>MNCVCRLVLVVLSLWPDTAVAPGPPPGPPRVSPDPRAELDSTVLLTRSLLADTRQLAAQLRDKFPADGDHNLDSLPTLAMSAGALGALQLPGVLTRLRADLLSYLRHVQWLRRAGGSSLKTLEPELGTLQARLDRLLRRLQLLMSRLALPQPPPDPPAPPLAPPSSAWGGIRAAHAILGGLHLTLDWAVRGLLLLKTRL[2x];>MSSSCSGLSRVLVAVATALVSASSPCPQAWGPPGVQYGQPGRSVKLCCPGVTAGDPVSWFRDGEPKLLQGPDSGLGHELVLAQADSTDEGTYICQTLDGALGGTVTLQLGYPPARPVVSCQAADYENFSCTWSPSQISGLPTRYLTSYRKKTVLGADSQRRSPSTGPWPCPQDPLGAARCVVHGAEFWSQYRINVTEVNPLGASTRLLDVSLQSILRPDPPQGLRVESVPGYPRRLRASWTYPASWPCQPHFLLKFRLQYRPAQHPAWSTVEPAGLEEVITDAVAGLPHAVRVSARDFLDAGTWSTWSPEAWGTPSTGTIPKEIPAWGQLHTQPEVEPQVDSPAPPRPSLQPHPRLLDHRDSVEQVAVLASLGILSFLGLVAGALALGLWLRLRRGGKDGSPKPGFLASVIPVDRRPGAPNL[2x];>[2x]MSAPRIWLAQALLFFLTTESIGQLLEPCGYIYPEFPVVQRGSNFTAICVLKEACLQHYYVNASYIVWKTNHAAVPREQVTVINRTTSSVTFTDVVLPSVQLTCNILSFGQIEQNVYGVTMLSGFPPDKPTNLTCIVNEGKNMLCQWDPGRETYLETNYTLKSEWATEKFPDCQSKHGTSCMVSYMPTYYVNIEVWVEAENALGKVSSESINFDPVDKVKPTPPYNLSVTNSEELSSILKLSWVSSGLGGLLDLKSDIQYRTKDASTWIQVPLEDTMSPRTSFTVQDLKPFTEYVFRIRSIKDSGKGYWSDWSEEASGTTYEDRPSRPPSFWYKTNPSHGQEYRSVRLIWKALPLSEANGKILDYEVILTQSKSVSQTYTVTGTELTVNLTNDRYVASLAARNKVGKSAAAVLTIPSPHVTAAYSVVNLKAFPKDNLLWVEWTPPPKPVSKYILEWCVLSENAPCVEDWQQEDATVNRTHLRGRLLESKCYQITVTLVFATGPGGSESLKAYLKQAAPARGPTVRTKKVGKNEAVLAWDQIPVDDQNGFIRNYSISYRTSVGKEMVVHVDSSHTEYTLSSLSSDTLYMVRMAAYTDEGGKDGPEFTFTTPKFAQGEIEAIVVPVCLAFLLTTLLGVLFCFNKRDLIKKHIWPNVPDPSKSHIAQWSPHTPPRHNFNSKDQMYSDGNFTDVSVVEIEANNKKPCPDDLKSVDLFKKEKVSTEGHSSGIGGSSCMSSSRPSISSNEENESAQSTASTVQYSTVVHSGYRHQVPSVQVFSRSESTQPLLDSEERPEDLQLVDSVDGGDEILPRQPYFKQNCSQPEACPEISHFERSNQVLSGNEEDFVRLKQQQVSDHISQPYGSEQRRLFQEGSTADALGTGADGQMERFESVGMETTIDEEIPKSYLPQTVRQGGYMPQ

The signalling receptor gp130 represents a paradigm for differential signal activation and functional diversity. It is required for interleukin (IL)−6, IL-11, IL-27, oncostatin-M (OSM), leukaemia inhibitory factor (LIF), ciliary neurotrophic factor (CNF), cardiotrophin-1 (CT-1), and cardiotrophin-like cytokine factor-1 (CLCF1) signalling. For IL-6 and IL-11 cytokines, gp130 signals by homodimerization of its intracellular domains. Similar to IL-6, IL-11 coordinates gp130 homodimers by forming a hexameric signalling complex comprised of two molecules each of gp130, IL-11 and co-receptor, IL-11Rα.

To understand how IL-11 instructs unique signalling outcomes through gp130, we solved the structure of the IL-11 receptor recognition complex by cryoEM. Complexes comprised two copies of the human IL-11 cytokine variant (IL-11 fused to domains D2 and D3 of IL-11Rα) and two copies of murine gp130P496L mutant (D1-D6), in agreement with a human IL-11 complex which came into press after submission of our manuscript. The final map was refined to a reported resolution of 3.1 Å using the gold standard FSC 0.143 cut-off; with local resolution ranging from 2.6 Å to 5.4 Å. IL-11 is a helical cytokine that coordinates a hexameric assembly with two copies of IL-11, IL-11Rα and gp130 through interactions at three principal binding sites. Site 1 of IL-11 is formed by the hinge between domains D2 and D3 of IL-11Rα. In our complex IL-11 residues T77-L90 are at an interface with IL-11Rα and adopt a helical conformation. A comparison with the crystal structure of apo IL-11 shows that these residues undergo a conformational change upon complex formation. We observe that for the IL-11 complex, the sidechain of IL-11:R135 at Site 2a inserts into a hydrophobic groove created by a hinge between domains D2 and D3 of gp130 (V190, W164, F169, Y184, I192, murine numbering). Here, IL-11Rα:R235 forms a salt bridge with gp130:E273. In the IL-11 complex, the Site 3a is comprised of a series of electrostatic interactions (gp130:K68-IL-11:D67, gp130:H71-IL-11:D62) and pi stacking between IL-11:W168 and gp130:Y116.>MRKIALFPGSFDPMTNGHLNLIERSAKLFDEVIIGVFINTSKQTLFTPEEKKYLIEEATKEMPNVRVIMQETQLTVESAKSLGANFLIRGIRNVKDYEYEKDIAKMNQHLAPEIETVFLLAEEPYAHVSSSLLKEVLRFGGDVSDYLPPNIYHALKQKK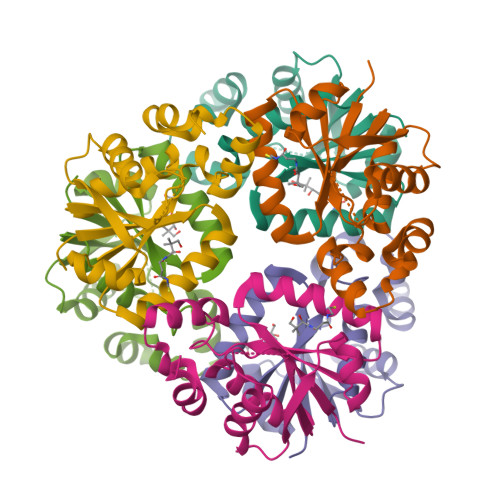NDWSLEHHHHHH[6x]>HTVSPVNPNAQQTTKTVMNWLAHLPNRTENRVLSGAFGGYSHDTFSMAEADRIRSATGQSPAIYGCDYARGWLETANIEDSIDVSCNSDLMSYWKNGGIPQISLHLANPAFQSGHFKTPITNDQYKKILDSSTAEGKRLNAMLSKIADGLQELENQGVPVLFRPLHEMNGEWFWWGLTSYNQKDNERISLYKQLYKKIYHYMTDTRGLDHLIWVYSPDANRDFKTDFYPGASYVDIVGLDAYFQDAYSINGYDQLTALNKPFAFTEVGPQTANGSFDYSLFINAIKQRYPKTIYFLAWNDEWSPAVNKGASALYHDSWTLNK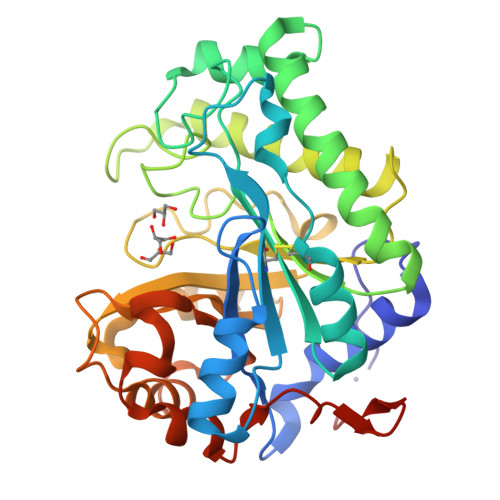GEIWNGDSLTPIVEHHHHHH[2x]> MSSPSKPTSPFVDDIEHESGSASNGLSSMSPFDDSFQFEKPSSAHGNIEVAKTGGSVLKRQSKPMKDISTPDLSKVTFDGIDDYSNDNDINDDDELNGKKTEIHEHENEVDDDLHSFQATPMPNTGGFEDVELDNNEGSNNDSQADHKLKRVRFGTRRNKSGRIDINRSKTLKWAKKNFHNAIDEFSTKEDSLENSALQNRSDELRTVYYNLPLPEDMLDEDGLPLAVYPRNKIRTTKYTPLTFFPKNILFQFHNFANIYFLILLILGAFQIFGVTNPGFASVPLIVIVIITAIKDGIEDSRRTVLDLEVNNTRTHILSGVKNENVAVDNVSLWRRFKKANTRALIKIFEYFSENLTAAGREKKLQKKREELRRKRNSRSFGPRGSLDSIGSYRMSADFGRPSLDYENLNQTMSQANRYNDGENLVDRTLQPNPECRFAKDYWKNVKVGDIVRVHNNDEIPADMILLSTSDVDGACYVETKNLDGETNLKVRQSLKCSKIIKSSRDITRTKFWVESEGPHANLYSYQGNFKWQDTQNGNIRNEPVNINNLLLRGCTLRNTKWAMGMVIFTGDDTKIMINAGVTPTKKSRISRELNFSVILNFVLLFILCFTAGIVNGVYYKQKPRSRDYFEFGTIGGSASTNGFVSFWVAVILYQSLVPISLYISVEIIKTAQAIFIYTDVLLYNAKLDYPCTPKSWNISDDLGQIEYIFSDKTGTLTQNVMEFKKCTINGVSYGRAYTEALAGLRKRQGVDVESEGRREKEEIAKDRETMIDELRSMSDNTQFCPEDLTFVSKEIVEDLKGSSGDHQQKCCEHFLLALALCHSVLVEPNKDDPKKLDIKAQSPDESALVSTARQLGYSFVGSSKSGLIVEIQGVQKEFQVLNVLEFNSSRKRMSCIIKIPGSTPKDEPKALLICKGADSVIYSRLDRTQNDATLLEKTALHLEEYATEGLRTLCLAQRELTWSEYERWVKTYDVAAASVTNREEELDKVTDVIERELILLGGTAIEDRLQDGVPDSIALLAEAGIKLWVLTGDKVETAINIGFSCNVLNNDMELLVVKASGEDVEEFGSDPIQVVNNLVTKYLREKFGMSGSEEELKEAKREHGLPQGNFAVIIDGDALKVALNGEEMRRKFLLLCKNCKAVLCCRVSPAQKAAVVKLVKKTLDVMTLAIGDGSNDVAMIQSADVGVGIAGEEGRQAVMCSDYAIGQFRYVTRLVLVHGKWCYKRLAEMIPQFFYKNVIFTLSLFWYGIYNNFDGSYLFEYTYLTFYNLAFTSVPVILLAVLDQDVSDTVSMLVPQLYRVGILRKEWNQTKFLWYMLDGVYQSVICFFFPYLAYHKNMVVTENGLGLDHRYFVGVFVTAIAVTSCNFYVFMEQYRWDWFCGLFICLSLAVFYGWTGIWTSSSSSNEFYKGAARVFAQPAYWAVLFVGVLFCLLPRFTIDCIRKIFYPKDIEIVREMWLRGDFDLYPQGYDPTDPSRPRINEIRPLTDFKEPISLDTHFDGVSHSQETIVTEEIPMSILNGEQGSRKGYRVSTTLERRDQLSPVTTTNNLPRRSMASARGNKLRTSLDRTREEMLANHQLDTRYSVERARASLDLPGINHAETLLSQRSRDR;> MVNFDLGQVGEVFRRKDKGAIVSGDNPEEEEDVDASEFEEDEVKPVRTKNRRPKEDAFTQQRLAAINPVLTPRTVLPLYLLIAVVFVIVGGCILAQNSKVDEVTIYYQDCMTNATSSWSDIPSEHWQFVFHKYKTYNTAPQWRFVDDESDDFTKQRGTCQIRFTTPSDMKNNVYLNYVLEKFAANHRRYVLSFSEDQIRGEDASYETVHDATGINCKPLSKNADGKIYYPCGLIANSMFNDTFPLQLTNVGDTSNNYSLTNKGINWESDKKRYKKTKYNYTQIAPPPYWEKMYPDGYNETNIPDIQDWEEFQNWMRPGAFDKITKLIRINKNDTLPAGEYQLDIGLHWPVLEFNGKKGIYLTHGSHLGGRNPFLGIVYLIGGCICAAMALILLTFWLFGGRKIADASSLSWNMK

P4 ATPases are involved in phospholipid translocation: they flip lipids from the extracellular side of the plasma membrane or from the lumenal side of internal organelles to the cytosolic side. Most P4 ATPases function as a heterodimeric complex: a catalytic α-subunit containing 10 transmembrane α-helices (TMHs) and a regulatory β-subunit of the Cdc50 (cell division cycle 50) protein family containing two TMHs. Dnf1 and Dnf2 share the same β-subunit, Lem3, and both are also capable of transporting PE and GlcCer. Here, we report the cryo-EM structures of Dnf1–Lem3 in three different states (E1, E1P-ADP, and E2P) and Dnf2–Lem3 in five different states (E1, E1-ATP, E1P-ADP, E2P, and E2P-transition).

There were Dnf1–Lem3 in the E1 (apo), E1P-ADP (AlF4−-ADP), and E2P (BeF3−) states; and Dnf2–Lem3 in the E1 (apo), E1-ATP (AMPPCP), E1P-ADP (ADP-AlF4−), E2P-transition (AlF4−), and E2P (BeF3−) states. Next, we performed single-particle cryo-EM on purified samples in apo form (E1 state) and on samples incubated with AMPPCP (E1-ATP state), AlF4−-ADP (E1P-ADP and E2P-transition states), or BeF3− (E2P state). During the subsequent phosphate (Pi) transition, when the enzyme changes from the E2P state to the E2P-transition state, the enzyme structure largely holds still; the 3D maps of Dnf2–Lem3 in these two states are nearly identical.>MGSSHHHHHHSSGLVPRGSHMGYSATAPVNLTRPATVPSMDGWTDGTGAWTLGEGTRVVSSDALAARAQSLASELTKFTDVDIKAATGSATGKDISLTLDASKKAELGDEGFKLNIGSKGLEVIGATDIGVFYGTRSVSQMLRQGQLTLPAGTVATKPKYKERGATLCACQINISTDWIDRFLSDMADLRLNYVLLEMKLKPEEDNTKKAATWSYYTRDDVKKFVKKANNYGIDVIPEINSPGHMNVWLENYPEYQLADNSGRKDPNKLDISNPEAVKFYKTLIDEYDGVFTTKYWHMGADEYMIGTSFDNYSKLKTFAEKQYGAGATPNDAFTGFINDIDKYVKAKGKQLRIWNDGIVNTKNVSLNKDIVIEYWYGAGRKPQELVQDGYTLMNATQALYWSRSAQVYKVNAARLYNNNWNVGTFDGGRQIDKNYDKLTGAKVSIWPDSSYFQTENEVEKEIFDGMRFISQMTWSDSRPWATWNDMKADIDKIGYPLDIREYDYTPVDAGIYDIPQLKSISKGPWELITTPDGYYQMKDTVSGKCLALFTGSKHLDVVTQVGARPELRNCADVSVGQDQRNTANERNTQKWQIRADKDGKYTISPALTQQRLAIATGNEQNI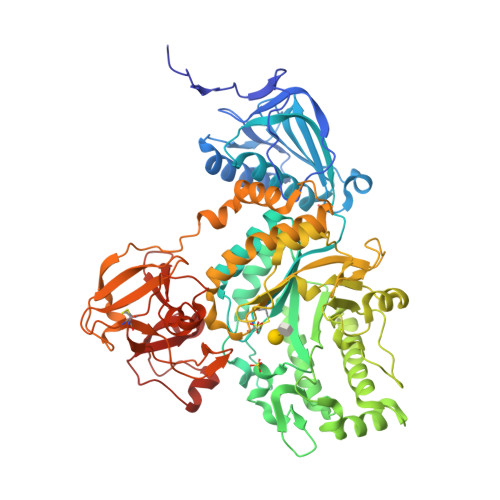DLETHRPAAGTVAQFPADLVSD[2x]> MTGIPTVTARPWTQRPRAENSTTNPTYFFTFGDSYSQTGFSASGTQPSASNPMGNPDLGIGTTTNGPNWIGYLTTTENASLVLSYNLAAGGATIDNALVPAWPGDLASQFRLFEDVYADKPASAPWSAEDAVFGVWIGINDIGNAYYSTDAETYTPKLISRLESLVEEVYKNGG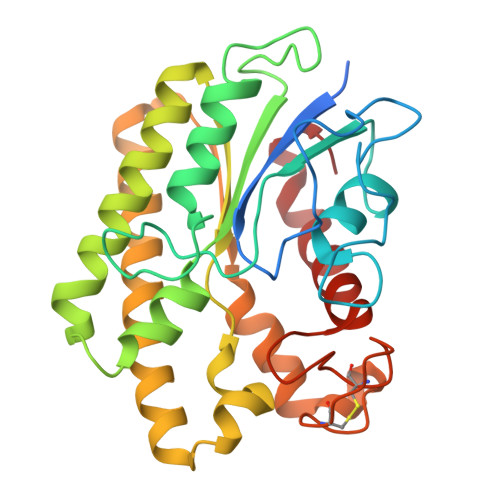RKFLFLNVPPTSRSPLFLEQGEEVVKQHAEYLSVYNENLEGMVDDFTKKKGDVTTVLYDSWSFMTKILDDPTAYGFPDATCINDDGTSCIWWDNYHPGMKYHLLQAEDMKPKLRKLGGW>[2x]GGUGCAGUAUUCUAGUCAGGGAAAUGCUUUUUGAAGGCGGGGCUAAAAAUCCGCUAAAGGGCACAUCGAUGAAGUUCCUGGUGCUGGCCUUAGAAUGCCCAGUCUUGGGCUUGUGCUGGGAGUUAAAAAAGCUGGGGCACUCGCAAUGGCAUGCGACAAAUGACCCUACUUUUGUGGAGGCCAAUUAUUGUAUAUUGAGAGAGAUAUUCAAUAUACGAAAUUGGGGUAAACCUGCAAUGUGGUGUAAAAGCUAUGUGCAGUGUAGCCUGCCUUGAGUGGUAUGGGGAGAGGAGAUAAACAAGUC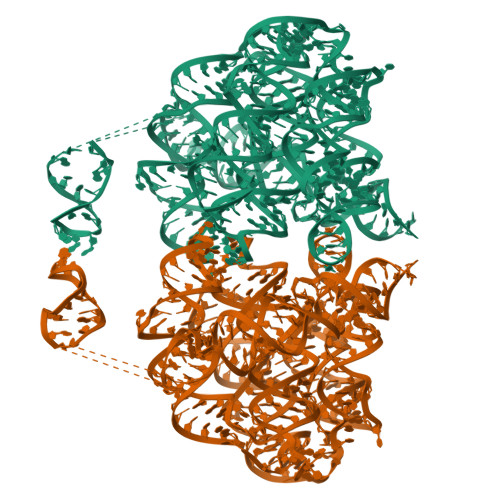AAAAAUUUUAGGCCUAAGUUUUUGUACUAUUGAACUCUGAAACCUAUGUUGCAAAAGAGGCUAAGAAAGCAUCUAACUGUUGAGGAAAACUCCUAGACUGUUUUGGUAAAAUGAGGAUUGCAGUGCGGACUUAGUGGCAAUUCAGUCCUGAAAGUGGCAACACUUCAGCUCGGAUAUUAAAGGGAAACCGCUAUAUGGCGACGUAUAGUUAUUCGUGGGGAAAGCCUACUGAACCUAUGCCGUAAGAUUUACUUAUUUUGUUACCACAUUGCC>[4x]MKRMLINATQQEELRVALVDGQRLYDLDIESPGHEQKKANIYKGKITRIEPSLEAAFVDYGAERHGFLPLKEIAREYFPANYSAHGRPNIKDVLREGQEVIVQIDKEERGNKGAALTTFISLAGSYLVLMPNNPRAGGISRRIEGDDRTELKEALASLELPEGMGLIVRTAGVGKSAEALQWDLSFRLKHWEAIKKAAESRPAPFLIHQESNVIVRAFRDYLRQDIGEILIDNPKVLELARQHIAALGRPDFSSKIKLYTGEIPLFSHYQIESQIESAFQREVRLPSGGSIVIDSTEALTAIDINSARATRGGDIEETAFNTNLEAADEIARQLRLRDLGGLIVIDFIDMTPVRHQRAVENRLREAVRQDRARIQISHISRFGLLEMSRQRLSPSLGESSHHVCPRCSGTGTVRDNESLSLSILRLIEEEALKENTQEVHAIVPVPIASYLLNEKRSAVNAIETRQDGVRCVIVPNDQMETPHYHVLRVRKGEETPTLSYMLPKLHEEAMALPSE

RNase E is an essential bacterial endoribonuclease involved in the turnover of messenger RNA and the maturation of structured RNA precursors in Escherichia coli. The N-terminal half forms the catalytic domain (residues 1–530), resembles its paralog RNase G, and is relatively conserved among prokaryotes (Marcaida et al., 2006). The RNase E catalytic domain forms a dimer of dimers, with a quaternary organization resembling two pairs of scissors arranged in tandem. Between these two domains is a pair of conserved CPxCxGxG motifs, one on each monomer, that coordinate a single zinc ion.

Here, we present the first crystal structure of the E. coli RNase E catalytic domain in the apo form at 3.3 Å resolution. The quaternary structure of the RNase E apoprotein is composed of a dimer-of-dimers connected via the small domains but has substantial deviations from the D2 symmetry observed in the holoprotein. Specifically, each is twisted by about 45° in the apoprotein relative to its orientation in the holoprotein, and the tetramer is bent out of the plane by ∼40°. Two zinc ions are present in the structure, one in each pocket. In each of the four apoprotein protomers, the combined S1 subdomain and 5′ sensor (from here on referred to collectively as the “5/S1 subdomain”) has moved as a single unit through an angle of about 60° relative to the holoprotein configuration. This conformational change significantly exposes both the binding and catalytic sites to the surrounding solvent and probably permits substrates to be more easily bound to the enzyme. Additional electron density was identified in the 5′ sensing pocket in three of the four monomers. On the basis of the coordination geometry and the buffer composition, we propose that this density is likely to be a sulfate ion. This ion is hydrogen-bonded to the T170 side chain and amide group, as well as to the R169 side chain, mimicking the interaction between RNase E and the 5′-monophosphate group of RNA seen in the holoprotein structure. In the structure presented here, these residues are oriented as in the previously reported holoprotein, but no electron density was apparent near the catalytic sites, suggesting that the metal may be absent.>SKPKQPPDASPANLLTSLVRAHLDSGPSTAKLDYSKFQELVLPHFGKEDAGDVQQFYDLLSGSLEVIRKWAEKIPGFAELSPADQDWLLESAFLELFILRLAYRSKPGEGKLIFCSGLVLHRLQCARGFGDWIDSILAFSRSLHSLLVDVPAFACLSALVLITDRHGLQEPRRVEELQNRIASCLKEHVAAVAGEPQPASCLSRLLGKLPELRTLCTQGLQRIFYLKLEDLVPPPP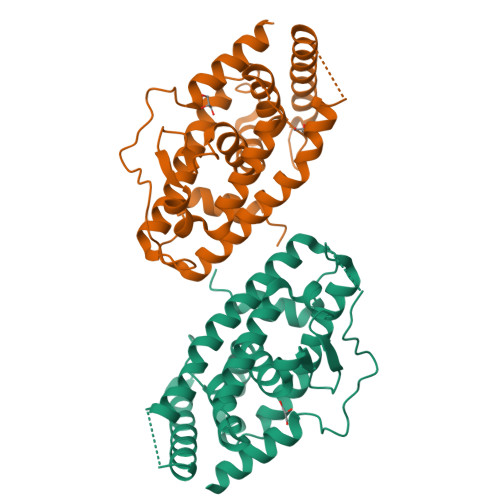IIDKIFMETLPFLEHHHHHH[2x]> LLQHVKFQSSNFENILTWDGGPASTSDTVYSVEYKKYGERKWLAKAGCQRITQKFCDLTMETRDHQEFYYAKVTAVSAGGPPVTKMTDRFSSLQHTTIKPPDVTCIPKVRSIQMLVHPTLTPVLSEDGHQLTLEEIFHDLFYRLELHVNHTYQMHLEGKQREYEFLGLT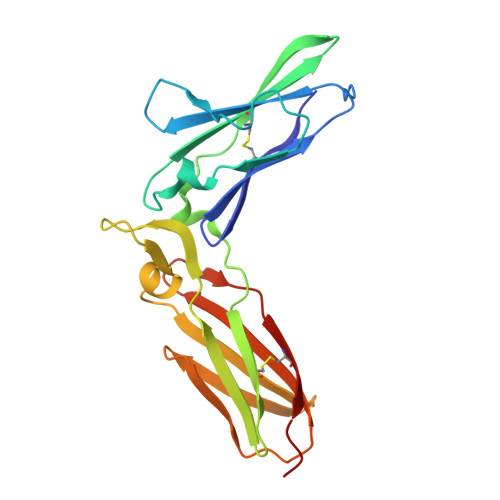PDTEFLGSITILTPILSKESAPYVCRVKTLPDGGS> AITTADNGNLHTWWHDNAVFNTTGPTGNDEVRRSSFYDLQVAQENQPDKAYDAFTYMSIPRSGKDKIGYTKEDGAEFSSQAGLTMSWSSFEYAKDVWVDVSLRTGQTITSADQVQIRPSSYNFEKQLVDADTVKIKVPYSDAGYRFSVEFEPQLYTAYNDMSGDSGKLTTEAEGNRAIHTEPRNSMMIFAEPKLRGEQKERLVPTEESGSIHYPAEGEVTNLNAVTEEIIYFKPGTYSMGSDYHAVLPPNVKWVYLAPGAYVKGAFRFLHDNQSQYKVTGYGVLSGEQYVYEADTNNNYNHLSGASNCHSSCVKMLQFASADAEQKLDLQGVTVAEPPYHSFVVYGNEQTFHMNVENYKQVGSWYWQTDGIELYKGSTMKNTFFNANDDVLKMYHSDVTIDNTVIWKNENGPVIQWGWTPRNIDNVNVTNTTVIHNRMYWKDVKYNTCILNSSSHWEDMGSTTKADPNTT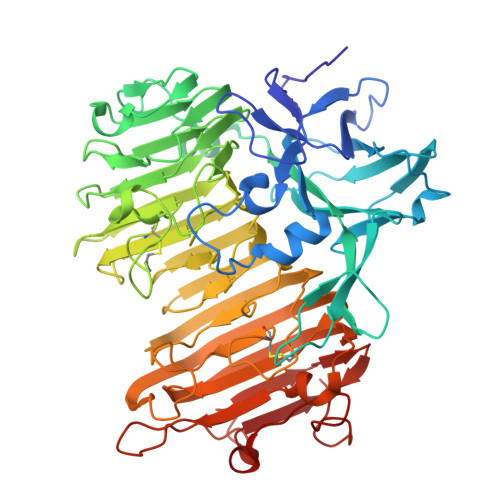VKNMRFENITVEGMTNCAIRVYALSDTENIHVKNLNIDAWNGLDWTSQVSHLKRYTNPAGEKVTIGNEIPDGNGLALENYSVGGEVIEKTADNWADHQLGRIGFDGENWNSWNAWRT> GMHPNIATLLSANLGESRTRHLLSLVSVPDGLPSDAEGRATRAEIAQALNMVLFAGILDRVPTGRAYTDDVAATGGKVVFDHGALRTVKWRDNGALPEGEAAFTRILRPLGYRLNGNYPLDRISMTGRSYAHADAPEGIAQFFVSEFHPERFSDAFREAVGRVTGNSADPLTPRAQTLLWQLDRDGVLTVADGAELIGLLVPCFERQHGVPRLADYETLLRESAEMAWIATEGNAFNHATDRVDDVFGLSEQQKALGRPMKDKVEVSGSGRVKQTAFRADTVRRQFIGAQGETVERDVPGSFYEFITRDRFADAPAASPRVDLGFDAGNAQGIFKMTA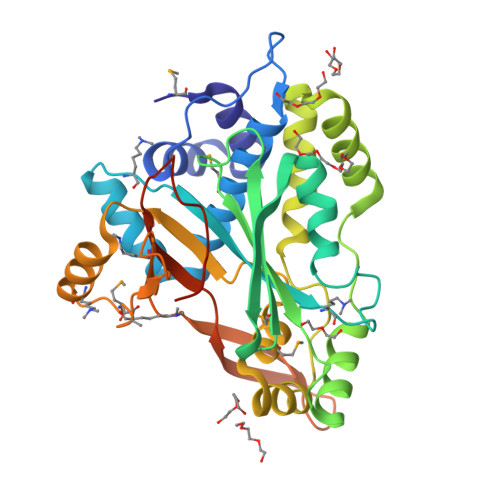AV>DKPVAHVVANHQVEEQLEWLSQRANALLANGMDLKDNQLVVPADGLYLVYSQVLFKGQGCPDYVLLTHTVSRFAISYQEKVNLLSAVKSPCPKDTPEGAELKPWYEPIYLGGVFQLEKGDQLSAEVNLPKYLDFAESGQVYFGVIAL[3x];>VCPQGKYIHPQDNSICCTKCHKGTYLYNDCPGPGQDTDCRECESGSFTASENHLRHCLSCSKCRKEMGQVEISSCTVDRDTVCGCRKNQYRHYWSENLFQCFNCSLCLNGTVHLSCQEKQNTVCTCHAGFFLRENECVSSSN[2x]

TNF, like most members of the TNF superfamily (TNFSF) exists mainly as a trimer with a threefold symmetry resulting in three identical receptor binding sites. The mechanism by which TNF induces signalling across the membrane is poorly understood, however, it is generally believed that the process involves receptor clustering. There are currently five approved TNF biologics that work by completely blocking the interaction of TNF with its receptors but to date, there are no small molecule therapeutics available that disrupt the high-affinity TNF–TNFR interaction. Small molecule inhibitors of TNF are described that stabilise a distorted TNF trimer, reducing the affinity of TNFR1 at one binding site and effectively reducing the stoichiometry of receptor binding from three to two per TNF trimer.

In order to further understand the impact of our compounds on receptor binding, we have crystallised mTNF with and without compound (UCB-4433) in complex with a truncated form of hTNFR1 (residues 41–184). The crystal structure of compound-bound mouse TNF (mTNF) in complex with humanTNFR1 (hTNFR1) reveals a distorted mTNF trimer with two copies of hTNFR1 bound. The degree of disruption of one of the receptor binding sites in the mTNF(UCB-4433)-TNFR1 structure was such that only two receptors were bound. Significantly, receptors that were bound were dimeric (described in detail below). In order to highlight the degree of distortion of the, arbitrarily defined, A–C receptor binding site, the UCB-4433 bound mTNF–hTNFR1 structure was compared with the complex without compound by aligning them through monomer C. Monomer A is twisted and tilted down and away from monomer C resulting in their partial separation. The degree of shift was measured for a number of amino acids that are involved in TNFR1 binding and the displacement ranged from 6.2 to 7.8 Å, making it impossible for the receptor to bridge across and bind the two monomers simultaneously, as observed at the two other binding sites. The individual monomers maintain their fold upon compound binding (RMSD of 0.5 Å), so the relevant positioning of residues involved in receptor binding within each individual monomer remains largely unchanged. It is, therefore, possible that receptor could still bind (albeit weakly) to either monomer A or C, however, this was not observed in the crystal structure suggesting that receptor binding prefers contact with adjacent monomers in the trimer to form a stable interaction.> GLVPRGSHMMEILRGSPALSAFRINKLLARFQAANLQVHNIYAEYVHFADLNAPLNDSEQAQLTRLLQYGPALSSHTPAGKLLLV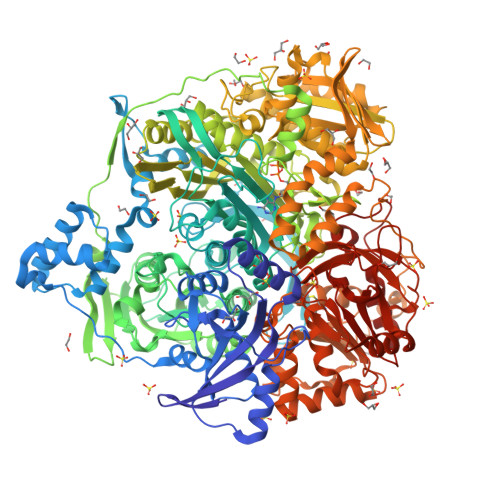TPRPGTISPWSSKATDIAHNCGLQQVDRLERGVAYYIEASTLTAEQWRQVAAELHDRMMETVFSSLTDAEKLFIHHQPAPVSSVDLLGEGRQALIDANLRLGLALAEDEIDYLQEAFTKLGRNPNDIELYMFAQANSEHCRHKIFNADWIIDGKPQPKSLFKMIKNTFETTPDYVLSAYKDNAAVMEGSAVGRYFADHNTGRYDFHQEPAHILMKVETHNHPTAISPWPGAATGSGGEIRDEGATGRGAKPKAGLVGFSVSNLRIPGFEQPWEEDFGKPERIVTALDIMTEGPLGGAAFNNEFGRPALTGYFRTYEEKVNSHNGEELRGYHKPIMLAGGIGNIRADHVQKGEIVVGAKLIVLGGPAMNIGLGAASSMASGQSDADLDFASVQRDNPEMERRCQEVIDRCWQLGDANPILFIHDVGAGGLSNAMPELVSDGGRGGKFELRDILSDEPGMSPLEIWCNESQERYVLAVAADQLPLFDELCKRERAPYAVIGDATEEQHLSLHDNHFDNQPIDLPLDVLLGKTPKMTRDVQTLKAKGDALNRADITIADAVKRVLHLPTVAEKTFLVTIGDRTVTGMVARDQMVGPWQVPVADCAVTTASLDSYYGEAMSIGERAPVALLDFAASARLAVGEALTNIAATQIGDIKRIKLSANWMAAAGHPGEDAGLYDAVKAVGEELCPQLGLTIPVGKDSMSMKTRWQEGNEQREMTSPLSLVISAFARVEDVRHTLTPQLSTEDNALLLIDLGKGHNALGATALAQVYRQLGDKPADVRDVAQLKGFYDAMQALVAARKLLAWHDRSDGGLLVTLAEMAFAGHCGVQVDIAALGDDHLAALFNEELGGVIQVRAEDRDAVEALLAQYGLADCVHYLGQALAGDRFVITANDQTVFSESRTTLRVWWAETTWQMQRLRDNPQCADQEHEAKANDTDPGLNVKLSFDINEDIAAPYIATGARPKVAVLREQGVNSHVEMAAAFHRAGFDAIDVHMSDLLGGRIGLGNFHALVACGGFSYGDVLGAGEGWAKSILFNHRVRDEFETFFHRPQTLALGVCNGCQMMSNLRELIPGSELWPRFVRNHSDRFEARFSLVEVTQSPSLLLQGMVGSQMPIAVSHGEGRVEVRDDAHLAALESKGLVALRYVDNFGKVTETYPANPNGSPNGITAVTTENGRVTIMMPHPERVFRTVANSWHPENWGEDSPWMRIFRNARKQLG>SGVGHSTGNYNNRTIFHYHGDEVTIICHATRHIHLNMSPTEEYKIYDTNHGPEFPNTGDQTQQGRNTVNDSYHAKVETPWYLINPNSWGIWFNPADFQQLITTCTHVTIETLTQEIDNIVIKTVSKQGSGAEETTQYNNDLTALLEVALDKSNMLPWVADNMYLNSLGYIPWRPCKLTQFCYHTNFYNTINLLEGTQQNQWSQIKEGIQYDNLQFTPIETSAEIDLLRTGDSWTSGTYHFKCKPTQLFYHWQSTRHIGAPHPTTSPEQEGQKGQIIQDTNGWQWGDRDNPISASTTVKDFHIGYSWPEWRWHYSTGGPSINPGSAFSQTPWGSEVGGTRLTQGASEKAIFDYNHGEAEPGHRDQWWQNNAQQTGQTNWAIKNAHQSELRNATASRETFWTQDYHNTFGPYTAVDDVGIQYPWGAMWGKQPDTTHKPMMSAHAPFTCQNGPPGQLLVKLAPNYTDSLNNEGLQTNRIVTFATFWWTGRCTFKAKLRTPRQFNAYQLPGIPSGTNPKKFVPDAIGRFELPFMPGRAMPNYTY[60x]

The BuVs, along with CuV and TuV belong to the genus Protoparvovirus, which prior the BuV discovery contained only animal (non-human) infecting viruses, and are classified as novel Primate protoparvovirus 1 species. The VP ORF encodes for two overlapping structural proteins, VP1 and VP2, sixty copies of which assemble their T = 1 icosahedral capsid in a predicted 1:10 ratio. The VP2 monomer extracted from the refined 60-mer capsids of the BuVs contained the core β-strands (βA–βI) and α-helix A (αA) observed in other parvoviruses and large loop insertions between these secondary structure elements. However, unlike the animal protoparvoviruses, the bufavirus capsid contain three separated protrusions surrounding the 3-fold axes, as has been reported for members of the Dependoparvovirus genus, human parvovirus B19, and the HBoVs.

Movie frame micrographs collected for these VLPs, at two different cryo-EM resources (West/Midwest Consortium for High-Resolution Cryo Electron Microscopy and SECM4) yielded capsid structures to 2.84, 3.79, and 3.25 Å resolution from 29,596, 7564, and 5234 particle images, respectively, for BuV1, BuV2, and BuV3. For each BuV, the first 32 N-terminal residues of VP2 were disordered, and thus residues modeled for BuV1, BuV2, and BuV3 were 33–568, 33–567, and 33–572, respectively, with the last residue being their C-terminus. In VR-I, two additional residues are inserted in BuV3 relative to BuV1 and BuV2 and VR-III contains conformational difference among all three BuV resulting in Cα position differences of up to 5.0 Å. VR-IX is mostly structurally conserved among all three viruses, with only the BuV2 residue 540 being conformationally different, VR-VI and VR-VII adopt different conformations, with BuV1 differing from BuV2 and BuV3 at VR-VI and BuV2 differing from BuV1 and BuV3 at VR-VII. The melting temperature (Tms) of the BuV capsids determined by DSF were 64.9 ± 0.2 °C for BuV1, 77.3 ± 0.3 °C for BuV2, and 73.4 ± 0.2 °C for BuV3. The Tm values obtained for BuV2 and BuV3 were within the range reported for other members of the protoparvovirus genus, for example, MVM. BuV1 contains five cysteine residues while BuV2 and BuV3 contain seven each. BuV3 does contain two cysteine residues, C59 and C520 within the same VP2 monomer, at a distance of 3.45 Å, positioned to interact within a hydrophobic pocket, but they are not engaged in a disulfide bond. This proximity may be contributing to the stable BuV3 phenotype compared to BuV1. Significantly, in all the structures determined to date for parvoviruses, either by X-ray crystallography or cryo-reconstruction, there has been no disulfide bond observed, despite the fact that cysteine residues have been positioned within interacting distance, similar to BuV3 C59 and C520.> GGRALRVLVNMDGVL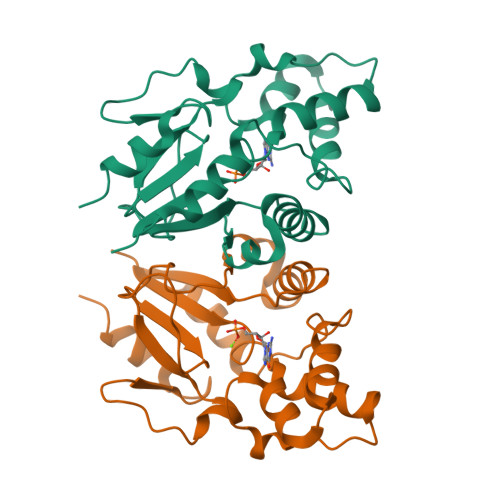ADFEGGFLRKFRARFPDQPFIALEDRRGFWVSEQYGRLRPGLSEKAISIWESKNFFFELEPLPGAVEAVKEMASLQNTDVFICTSPIKMFKYCPYEKYAWVEKYFGPDFLEQIVLTRDKTVVSADLLIDDRPDITGAEPTPSWEHVLFTACHNQHLQLQPPRRRLHSWADDWKAILDSKRPC>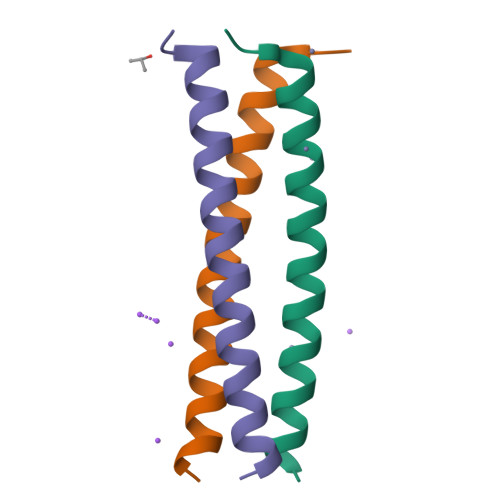DVDIETLKQELLELKQRYEAQQKALAVLEQRVRQVEDQ[6x]>MSKDYQSLAKLSPFELKDELIKIASSDGNRLMLNAGRGNPNFLATTPRRAFFRLGLFAAAESELSYSYMTTVGVGGLAKIDGIEGRFERYIAENRDQEGVRFLGKSLSYVRDQLGLDPAAFLHEMVDGILGCNYPVPPRMLNISEKIVRQYII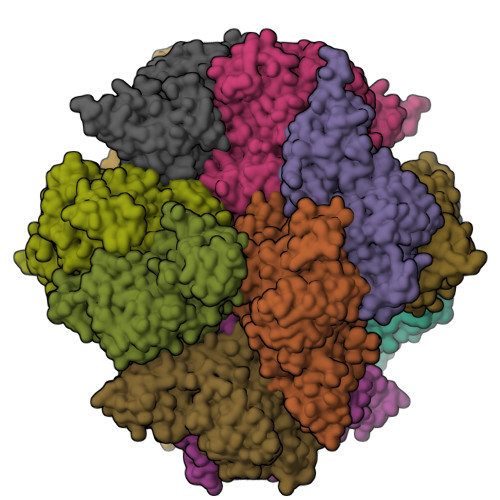REMGADAIPSESVNLFAVEGGTAAMAYIFESLKLNGLLKAGDKVAIGMPVFTPYIEIPELAQYALEEVAINADPSLNWQYPDSELDKLKDPAIKIFFCVNPSNPPSVKMDQRSLERVRNIVAEHRPDLMILTDDVYGTFADDFQSLFAICPENTLLVYSFSKYFGATGWRLGVVAAHQQNVFDLALDKLQESEKVALDHRYRSLLPDVRSLKFIDRLVADSRAVALNHTAGLSTPQQVQMALFSLFALMDEADEYKHTLKQLIRRRETTLYRELGMPPLRDENAVDYYTLIDLQDVTAKLYGEAFSEWAVKQSSTGDMLFRIADETGIVLLPGRGFGSNRPSGRASLANLNEYEYAAIGRALRKMADELYAEYSGQAQNLKLAAALEHHHHHH[6x]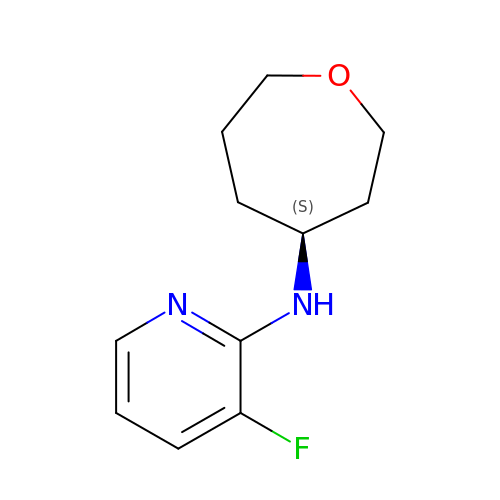3-fluoro-N-[(4S)-oxepan-4-yl]pyridin-2-amine | C11 H15 F N2 O | NXRZJDZFJRRYPW-VIFPVBQESA-N> MKKKVLIGASLAAVVLTGAAMVGAAVPPPPVNQFLGIYDTKFPNLTKADCLECHVSDTVLVQQHHALINTVTPPASCINTSGTVPPTLATGCHVMVPDGSGGFTFQDFRNCFNCHTQTPHHTSPAAVAKDCKYCHGNFIDNPLDGHYIPTYSASSVTPMPSGRSVTATDGNVVIVQGCEACHQAAPNAIDPKTNTVRPIFSNQDTHHGTGITDCNLCHNTSSNVPIRQCEVCHGVNSLHNIQKDSPNAANLGTVKPGLEDLGWGHIGNNWDCQGCHWSWFGNSSPYTNATVPAINGQSSYTVTAGKEAVLTIVGSSFVNVGPDGVT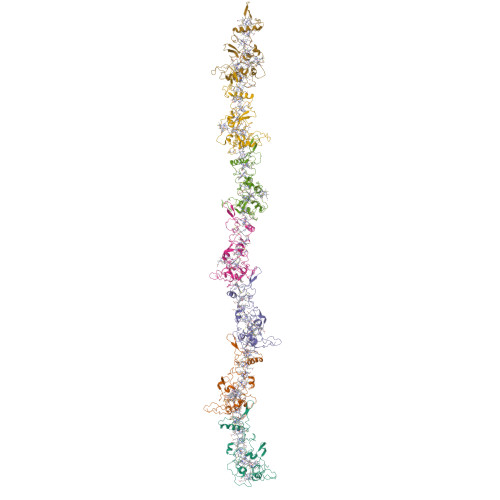TYQPTVALVSGSTSLTLTPFSVTESEIKVSVPALVEGVYELRITKANKVSNLAKLTVAPARIIASATLATGKTLTITGTGFGPAPSSEYDAGIGVYAGTTQANVISWSDTKVVATSPDFATNGYVTVKTINGPLSGKILAAPKKVKR> MVREFLAEFMSTYVMMVFGLGSVAHMVLNKKYGSYLGVNL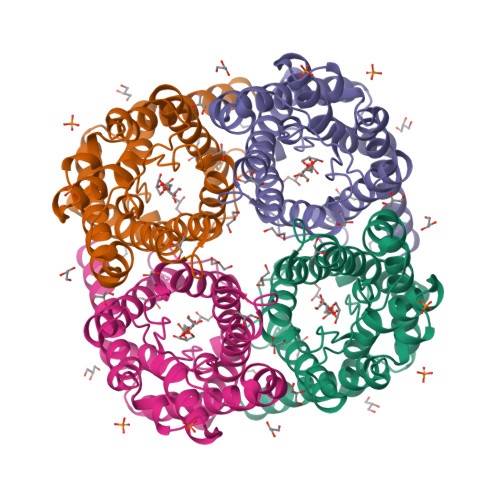GFGFGVTMGVHVAGRISGAHMNAAVTFANCALGRVPWRKFPVYVLGQFLGSFLAAATIYSLFYTAILHFSGGQLMVTGPVATAGIFATYLPDHMTLWRGFLNEAWLTGMLQLCLFAITDQENNPALPGTEALVIGILVVIIGVSLGMNTGYAINPSRDLPPRIFTFIAGWGKQVFSNGENWWWVPVVAPLLGAYLGGIIYLVFIGST>[2x]MRGSHHHHHHGSELSIPELRERIKNVAEKTLEDEVKSLSLDEVIGEIIDLELDDQAISILEIKQEHVFSRNQIARGHHLFAQANSLAVAVI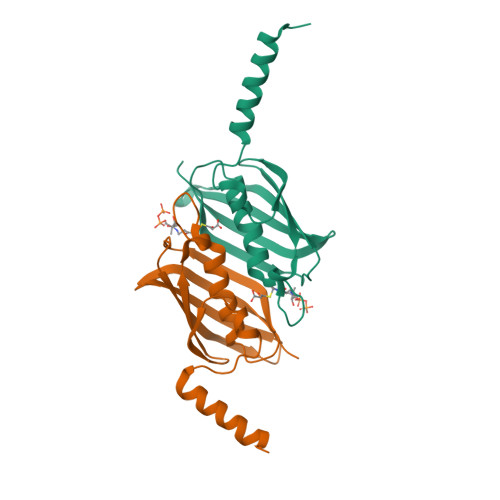DDELALTASADIRFTRQVKQGERVVAKAKVTAVEKEKGRTVVEVNSYVGEEIVFSGRFDMYRSKHS>[6x]SMGFWEASSRGGGAFSGGEDASEGGAEEGAGGAGGSAGAGEGPVITALTPMTIPDVFPHLPLIAITRNPVFPRFIKIIEVKNKKLVELLRRKVRLAQPYVGVFLKRDDSNESDVVESLDEIYHTGTFAQIHEMQDLGDKLRMIVMGHRRVHISRQLEVEPEEPEAENKHKPRRKSKRGKKEAEDELSARHPAELAMEPTPELPAEVLMVEVENVVHEDFQVTEEVKALTAEIVKTIRDIIALNPLYRESVLQMMQAGQRVVDNPIYLSDMGAALTGAESHELQDVLEETNIPKRLYKALSLLKKEFELSKLQQRLGREVEEKIKQTHRKYLLQEQLKIIKKELGLEKDDKDAIEEKFRERLKELVVPKHVMDVVDEELSKLGLLDNHSSEFNVTRNYLDWLTSIPWGKYSNENLDLARAQAVLEEDHYGMEDVKKRILEFIAVSQLRGSTQGKILCFYGPPGVGKTSIARSIARALNREYFRFSVGGMTDVAEIKGHRRTYVGAMPGKIIQCLKKTKTENPLILIDEVDKIGRGYQGDPSSALLELLDPEQNANFLDHYLDVPVDLSKVLFICTANVTDTIPEPLRDRMEMINVSGYVAQEKLAIAERYLVPQARALCGLDESKAKLSSDVLTLLIKQYCRESGVRNLQKQVEKVLRKSAYKIVSGEAESVEVTPENLQDFVGKPVFTVERMYDVTPPGVVMGLAWTAMGGSTLFVETSLRRPQDKDAKGDKDGSLEVTGQLGEVMKESARIAYTFARAFLMQHAPANDYLVTSHIHLHVPEGATPKDGPSAGCTIVTALLSLAMGRPVRQNLAMTGEVSLTGKILPVGGIKEKTIAAKRAGVTCIVLPAENKKDFYDLAAFITEGLEVHFVEHYREIFDIAFPD

The hexameric, barrel-forming, AAA+ protease Lon is critical for maintaining mitochondrial matrix protein homeostasis. A human Lon monomer contains a mitochondrial targeting sequence, a Lon-associated N-terminal (LAN) domain, an α-helical neck region, an AAA+ domain, and a protease domain (PD) in a single chain. The LAN domains specifically recognize and capture fully or partially unfolded substrates, which are then threaded towards the barrel chamber for degradation using the chemical energy from ATP hydrolysis. We determined high-resolution structures of substrate-engaged, substrate-trapped, and substrate-free forms of the human mitochondrial Lon protease.

The Lon^SE^ map shows additional density in the barrel pore that we attributed to a substrate peptide ([Fig fig1]; [Fig fig2]). The substrate side chains are not resolved, probably due to averaging different substrates during single-particle reconstruction, and therefore a polyalanine sequence was modelled. The substrate is contacted by two pore loops (termed pore loop 1 and 2) in P1–P3 but is contacted only by pore loop 1 in P4 and pore loop 2 in P5. The substrate is not contacted at all by P6 (seam protomer, [Fig fig2]). The final modelled substrate is 11 residues long and adopts a twisted β-strand conformation that follows the right-handed helical arrangement of the pore loops. Taken together, the pore loops in Lon^SE^ have a right-handed staircase arrangement around the central vertical axis of the chamber. Lon^SE^ P4 and P5 are ADP-bound, while the “seam” protomer P6 is ATP-bound. For the Lon^SE^ protomers with bound ATP/ATP’ (P1–P3, P6) the AAA+-domains are located further from their respective PD in comparison to the AAA+-domains in the protomers with bound ADP. Therefore, the Lon^SE^ structure presented here represents the stage immediately following nucleotide exchange in the seam protomer P6, and prior to its re-engagement in substrate binding. Consistent with Lon^SE^ being in an active conformation, the PDs display in-plane six-fold symmetry and an open gate loop.>[2x]GAEIPK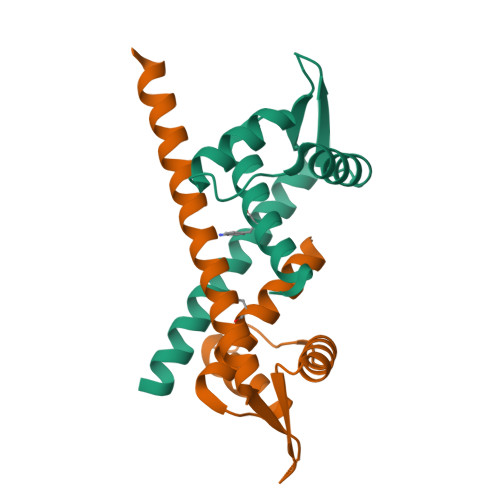EMLRAQTNXILRNVLKQGDNYVYGIIKQVKEASNGEMELNEATLYTIFKRLEKDGIISSYWGDESQGGRRKYYRLTEIGHENNRLAFEGWSRVDKIIENLEANKKSEAIKSRWSHPQFEK N-[(R)-1-benzofuran-2-yl(phenyl)methyl]-3,4-dihydro-2H-1,5-benzodioxepine-7-sulfonamide | C24 H21 N O5 S | 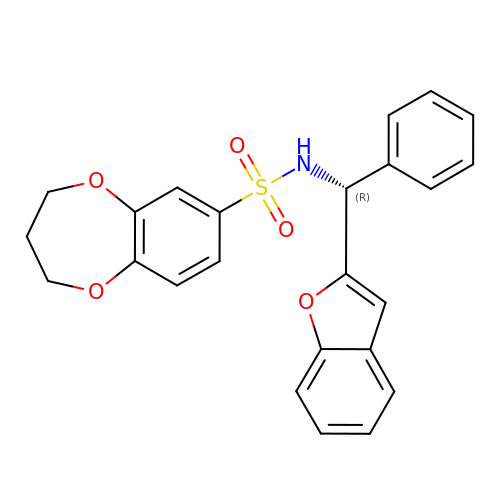KMUUQMAWJDDNPP-XMMPIXPASA-N1-BROMOPROPANE | 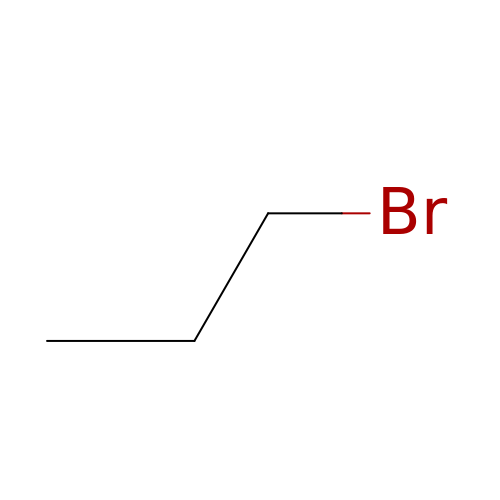C3 H7 Br | CYNYIHKIEHGYOZ-UHFFFAOYSA-N5'-O-[(3-cyanobenzene-1-carbonyl)sulfamoyl]adenosine | C18 H17 N7 O7 S | 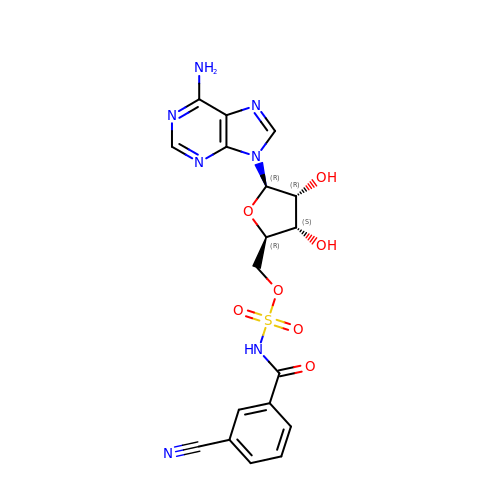MLNMSDSFICXLTI-XWXWGSFUSA-N> MSLGVLAAAIAVGLGALGAGIGNGLIVSRTIEGIARQPELRPVLQTTMFIG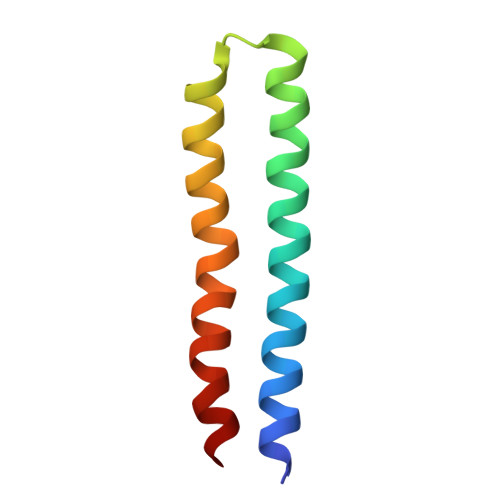VALVEALPIIGVVFSFIYLGR>[2x]HMASKMFFINDETPWEELGNGIKRKVMTWSDDLMMVCVHFDKGAIGVAHKHDIHDQIAYVAAGSFEVEIEGQKRILKAGDAYRAVKNEMHG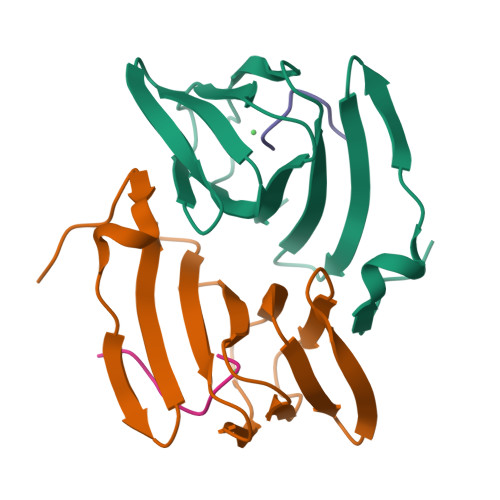AVSLEDNSILIDTFNPKRDDFL;>GSSHHHHH[2x]> MMRRVYSPVFCSVAAARFAATSAAKKYDLFGYEVDTNTAPWIEKIKKCKYYDEAGEVLVNMNVSNCPPDIATYNATLQCIYQSPSKQ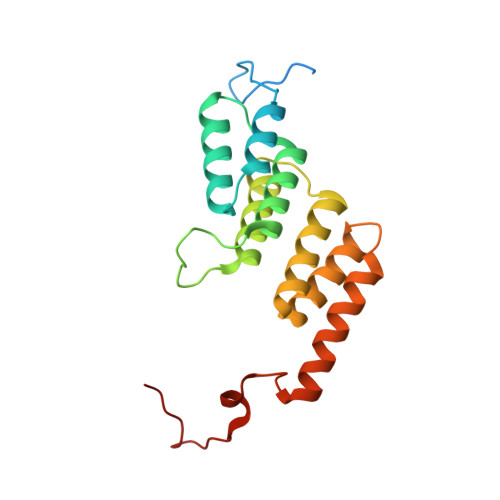STPVDNESKFCAMMDLLEEMQHRNRLKPNEESWTWVMKECVKSGQFRLGYCIQQVMETECKGCPADLVKANEANAQKAKTEGKEHPGHLSQQAGLFDVKVE> GPLGSLELSRREFVFENVKFRQLQKEKFQISNNGQVPCHFSFIPKLNDSQYCKPWLRAEPFEGYLEPNETVDISLDVYVSKDSVTILNSGEDKIEDILVLHLDRGKDYFLTISGNYLPSCFGTSLEALCRMKRPIREVPVTKLIDLEEDSFLEKEKSLLQMVPLDEGASERPLQVPKEIWLLVDHLFKYACHQEDLFQTPGMQEELQ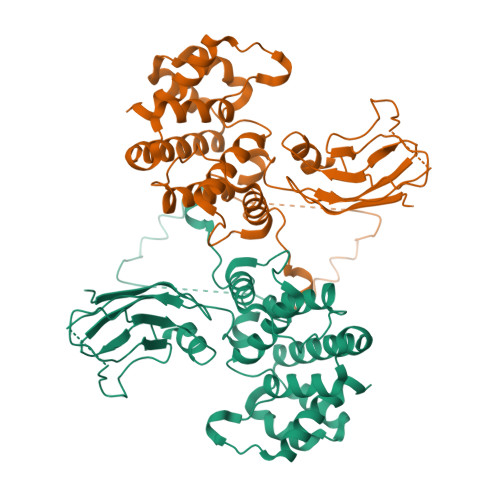QIIDCLDTSIPETIPGSNHSVAEALLIFLEALPEPVICYELYQRCLDSAYDPRICRQVISQLPRCHRNVFRYLMAFLRELLKFSEYNSVNANMIATLFTSLLLRPPPNLMARQTPSDRQRAIQFLLGFLLGSEED> GSMHMQLEEI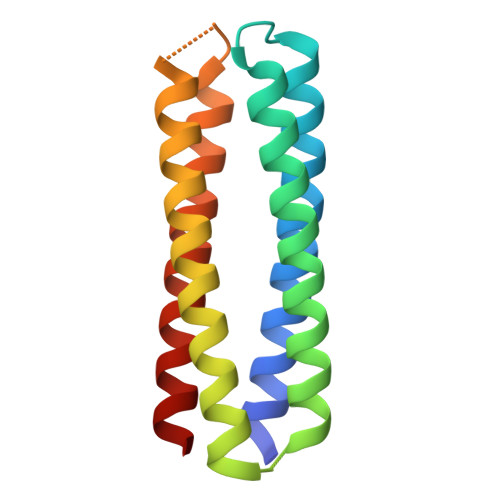AQQLEEIAKQLKKIAWQLKKIAQGEPSAQGQLEEIAQQLEEIAKQLKKIAWQLKKIAQGPDSVQLEEIAQQLEEIAKQLKKIAWQLKKIAQGGTSGGQLEEIAQQLEEIAKQLKKIAWQLKKIAQ(2R)-2-{[(S)-[(1R)-1-amino-3-methylbutyl](hydroxy)phosphoryl]methyl}pentanedioic 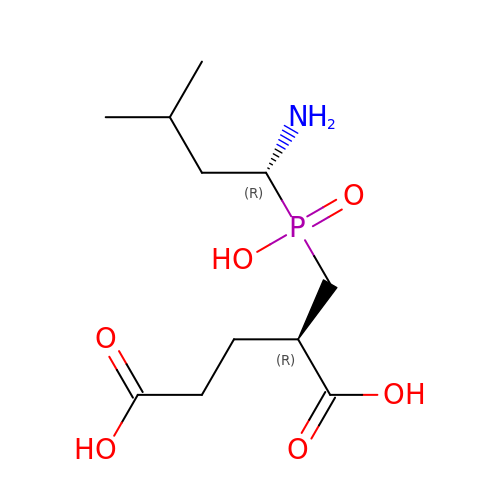acid | C11 H22 N O6 P | GANKYZVDRZVCGT-DTWKUNHWSA-N> HVFIRTELSFIKNNVPCIRDMFFIYKRELYNICLDDLKGEEDETHIYVQKKVKDSWITLNDLFKETDLTGRPHIFAYVDVEEIIILLCEDEEFSNRKKDMTCHRFYSNDGKEYQNSEITISDYILKDKLLSSYVSLPLKIENREYFLICGVSPYKFK;> HVFIRTELSFIKNNVPCIRDMFFIYKRELYNICLDDLKGEEDETHIYVQKKVKDSWITLNDLFKETDLTGRPHIFAYVDVEEIIILLCEDDEFSNRKKDMTCHRFYSNDGKEYQNSEITISDYILKDKLLSSYVSLPLKIENREYFLICGVSPYKFKDDNK;> DDNKKDDILCMASHDKGETWGTKIVIKYDNYKLGVQYFFLRPYISKNDLSFHFYVGDNINNVKNVNFIECTHEKDLEFVCSNRDFLKDNKVLQDVSTLNDEYIVSYGNDNNFAECYIFFNNENSILIKPEKYGQTTAGCYGGTFVKIDEQRTLFIYSS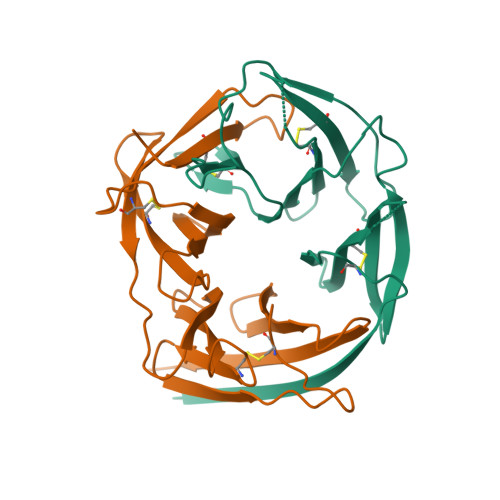SQGIYNIHTIYYANYEEF;> KDDILCMASHDKGETWGTKIVIKYDNYKLGVQYFFLRPYISKNDLSFHFYVGDNINNVKNVNFIECTHEKDLEFVCSNRDFLKDNKVLQDVSTLNDEYIVSYGNDNNFAECYIFFNNENSILIKPEKYGNTTAGCYGGTFVKIDEQRTLFIYSSSQGIYNIHTIYYANYE> QSEPELKLESVVIVSRHGVRAPTKATQLMQDVTPDAWPTWPVKLGWLTPRGGELIAYLGHYQRQRLVADGLLAKKGCPQSGQVAIIADTDERTRKTGEAFAAGLAPDCAITVHTQVDTSSPDPLFNPLKTGVCQLDNANVTDAILSRAGGSIADFTGHRQTAFRELERVLNFPQSNLCLKREKQDESCSLTQALPSELKVSADNVALTGAVSLASMLTEIFLLQQAQGMPEPGWGRITDSHQWNTLLSLHNAQFYLLQRTPEVARSR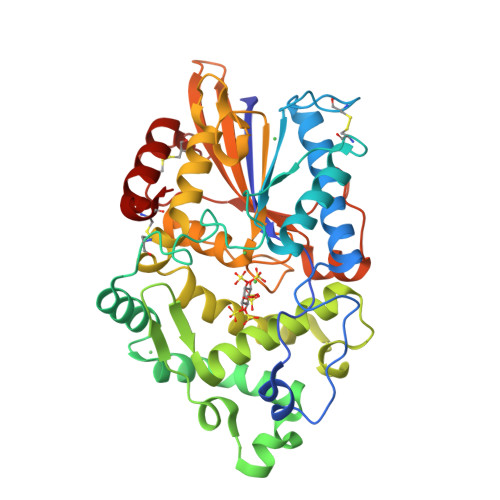ATPLLDLIKTALTPHPPQKQAYGVTLPTSVLFIAGHDTNLANLGGALELNWTLPGQPDNTPPGGELVFERWRRLSDNSQWIQVSLVFQTLQQMRDKTPLSLNTPPGEVKLTLAGCEERNAQGMCSLAGFTQIVNEARIPACSL SF3B1 is a central component of the SF3b subcomplex in the U2 small nuclear RNP (snRNP) and plays a pivotal role in the early stages of spliceosome assembly and branch point adenosine (BPA) recognition (Gozani et al. 1998). SF3B1 is intimately associated with three other proteins: PHF5A, SF3B3, and SF3B5. SF3B1 is composed of some 20 HEAT repeats that form a superhelical spiral of one turn that wraps around PHF5A. SF3B1, part of the U2 small nuclear RNP (snRNP), is targeted by splicing modulators, including E7107, the first to enter clinical trials, and, more recently, H3B-8800.

Here, we present the cryogenic electron microscopy (cryo-EM) structure of the SF3b subcomplex (SF3B1, SF3B3, PHF5A, and SF3B5) bound to E7107 at 3.95 Å. The cryo-EM map shows that E7107 binds at the interface of SF3B1 and PHF5A. SF3B1 encircles PHF5A and, at the interface of the HEAT repeats 15–17, forms a deep channel from the top to the bottom face, where the BPA binds. E7107 fills this channel like a plug. Residues V1110, V1114, L1066, and V1078 from SF3B1 and residue Y36 from PHF5A make interactions with the compound. The macrocycle is positioned in part by the interactions with positive-charged residues R1074, R1075, and K1071 of SF3B1 at the periphery of the channel. The cycloheptyl-piperazine is sandwiched between SF3B1Y1157 and PH5AR38. SF3B1R1074H and PHF5AY36C mutations confer the strongest levels of resistance (>500-fold). Both residues sit deep in the binding pocket on orthogonal sides and are situated adjacent to the diene tail of E7107. Our cryo-EM structure bound to E7107 shows that SF3B1 closely resembles the open conformation. Moreover, superposition of our E7107-bound structure with the RNA-bound structure from Bact shows that the diene tail region of E7107 would clash with the BPA.

> DMFLYNLTLQRATGISFAIHGNFSGTKQQEIVVSRGKILELLRPDPNTGKVHTLLTVEVFGVIRSLMAFRLTGGTKDYIVVGSDSGRIVILEYQPSKNMFEKIHQETFGKSGCRRIVPGQFLAVDPKGRAVMISAIEKQKLVYILNRDAAARLTISSPLEAHKANTLVYHVVGVDVGFENPMFACLEMDYEEADNDPTGEAAANTQQTLTFYELDLGLNHVVRKYSEPLEEHGNFLITVPGGSDGPSGVLICSENYITYKNFGDQPDIRCPIPRRRNDLDDPERGMIFVCSATHKTKSMFFFLAQTEQGDIFKITLETDEDMVTEIRLKYFDTVPVAAAMCVLKTGFLFVASEFGNHYLYQIAHLGDDDEEPEFSSAMPLEEGDTFFFQPRPLKNLVLVDELDSLSPILFCQIADLANEDTPQLYVACGRGPRSSLRVLRHGLEVSEMAVSELPGNPNAVWTVRRHIEDEFDAYIIVSFVNATLVLSIGETVEEVTDSGFLGTTPTLSCSLLGDDALVQVYPDGIRHIRADKRVNEWKTPGKKTIVKCAVNQRQVVIALTGGELVYFEMDPSGQLNEYTERKEMSADVVCMSLANVPPGEQRSRFLAVGLVDNTVRIISLDPSDCLQPLSMQALPAQPESLCIVEMGGTEKQDELGERGSIGFLYLNIGLQNGVLLRTVLDPVTGDLSDTRTRYLGSRPVKLFRVRMQGQEAVLAMSSRSWLSYSYQSRFHLTPLSYETLEFASGFASEQCPEGIVAISTNTLRILALEKLGAVFNQVAFPLQYTPRKFVIHPESNNLIIIETDHNAYTEATKAQRKQQMAEEMVEAAGEDERELAAEMAAAFLNENLPESIFGAPKAGNGQWASVIRVMNPIQGNTLDLVQLEQNEAAFSVAVCRFSNTGEDWYVLVGVAKDLILNPRSVAGGFVYTYKLVNNGEKLEFLHKTPVEEVPAAIAPFQGRVLIGVGKLLRVYDLGKKKLLRKCENKHIANYISGIQTIGHRVIVSDVQESFIWVRYKRNENQLIIFADDTYPRWVTTASLLDYDTVAGADKFGNICVVRLPPNTNDEVDEDPTGNKALWDRGLLNGASQKAEVIMNYHVGETVLSLQKTTLIPGGSESLVYTTLSGGIGILVPFTSHEDHDFFQHVEMHLRSEHPPLCGRDHLSFRSYYFPVKNVIDGDLCEQFNSMEPNKQKNVSEELDRTPPEVSKKLEDIRTRYAFDYKDD;> MTDRYTIHSQLEHLQSKYIGTGHADTTKWEWLVNQHRDSYCSYMGHFDLLNYFAIAENESKARVRFNLMEKMLQPCGPPADKPEEN;> MAKIAKTHEDIEAQIREIQGKKAALDEAQGVGLDSTGYYDQEIYGGSDSRFAGYVTSIAATELEDDDDDYSSSTSLLGQKKPGYHAPVALLNDIPQSTEQYDPFAEHRPPKIADREDEYKKHRRTMIISPERLDPFADGGKTPDPKMNARTYMDVMREQHLTKEEREIRQQLAEKAKAGELKVVNGAAASQPPSKRKRRWDQTADQTPGATPKKLSSWDQAETPGHTPSLRWDETPGRAKGSETPGATPGSKIWDPTPSHTPAGAATPGRGDTPGHATPGHGGATSSARKNRWDETPKTERDTPGHGSGWAETPRTDRGGDSIGETPTPGASKRKSRWDETPASQMGGSTPVLTPGKTPIGTPAMNMATPTPGHIMSMTPEQLQAWRWEREIDERNRPLSDEELDAMFPEGYKVLPPPAGYVPIRTPARKLTATPTPLGGMTGFHMQTEDRTMKSVNDQPSGNLPFLKPDDIQYFDKLLVDVDESTLSPEEQKERKIMKLLLKIKNGTPPMRKAALRQITDKAREFGAGPLFNQILPLLMSPTLEDQERHLLVKVIDRILYKLDDLVRPYVHKILVVIEPLLIDEDYYARVEGREIISNLAKAAGLATMISTMRPDIDNMDEYVRNTTARAFAVVASALGIPSLLPFLKAVCKSKKSWQARHTGIKIVQQIAILMGCAILPHLRSLVEIIEHGLVDEQQKVRTISALAIAALAEAATPYGIESFDSVLKPLWKGIRQHRGKGLAAFLKAIGYLIPLMDAEYANYYTREVMLILIREFQSPDEEMKKIVLKVVKQCCGTDGVEANYIKTEILPPFFKHFWQHRMALDRRNYRQLVDTTVELANKVGAAEIISRIVDDLKDEAEQYRKMVMETIEKIMGNLGAADIDHKLEEQLIDGILYAFQEQTTEDSVMLNGFGTVVNALGKRVKPYLPQICGTVLWRLNNKSAKVRQQAADLISRTAVVMKTCQEEKLMGHLGVVLYEYLGEEYPEVLGSILGALKAIVNVIGMHKMTPPIKDLLPRLTPILKNRHEKVQENCIDLVGRIADRGAEYVSAREWMRICFELLELLKAHKKAIRRATVNTFGYIAKAIGPHDVLATLLNNLKVQERQNRVCTTVAIAIVAETCSPFTVLPALMNEYRVPELNVQNGVLKSLSFLFEYIGEMGKDYIYAVTPLLEDALMDRDLVHRQTASAVVQHMSLGVYGFGCEDSLNHLLNYVWPNVFETSPHVIQAVMGALEGLRVAIGPCRMLQYCLQGLFHPARKVRDVYWKIYNSIYIGSQDALIAHYPRIYNDDKNTYIRYELDYIL;> DLIFCRKQAGVAIGRLCEKCDGKCVICDSYVRPCTLVRICDECNYGSYQGRCVICGGPGVSDAYYCKECTIQEKDRDGCPKIVNL>[3x]GTNS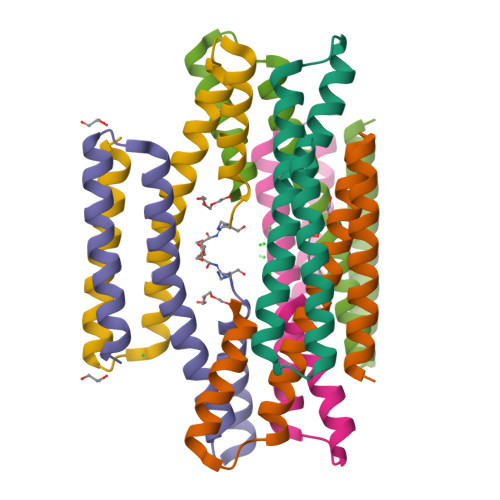KYITALKRSEGQLRGIQKMIEGDRDCADIVTQLTAVRSSVERVIEMIITENLTECINQPLDDSEAQKERLEKAIRYLIKRK> TA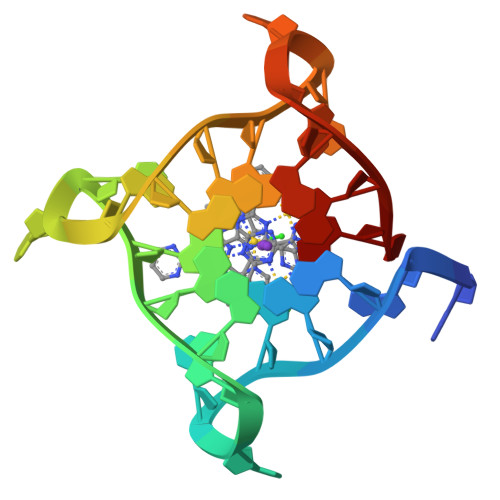GGGTTAGGGTTAGGGTTAGGGT> MASSRCPAPRGCRCLPGASLAWLGTVLLLLADWVLLRTALPRIFSLLVPTALPLLRVWAVGLSRWAVLWLGACGVLRATVGSKSENAGAQGWLAALKPLAAALGLALPGLALFRELISWGAPGSADSTRLLHWGSHPTAFVVSYAAALPAAALWHKLGSLWVPGGQGGSGNPVRRLLGCLGSETRRLSLFLVLVVLSSLGEMAIPFFTGRLTDWILQDGSADTFTRNLTLMSILTIASAVLEFVGDGIYNNTMGHVHSHLQGEVFGAVLRQETEFFQQNQTGNIMSRVTEDTSTLSDSLSENLSLFLWYLVRGLCLLGIMLWGSVSLTMVTLITLPLLFLLPKKVGKWYQLLEVQVRESLAKSSQVAIEALSAMPTVRSFANEEGEAQKFREKLQEIKTLNQKEAVAYAVNSWTTSISGMLLKVGILYIGGQLVTSGAVSSGNLVTFVLYQMQFTQAVEVLLSIYPRVQKAVGSSEKIFEYLDRTPRCPPSGLLTPLHLEGLVQFQDVSFAYPNRPDVLVLQGLTFTLRPGEVTALVGPNGSGKSTVAALLQNLYQPTGGQLLLDGKPLPQYEHRYLHRQVAAVGQEPQVFGRSLQENIAYGLTQKPTMEEITAAAVKSGAHSFISGLPQGYDTEVDEAGSQLSGGQRQAVALARALIRKPCVLILDDATSALDANSQLQVEQLLYESPERYSRSVLLITQHLSLVEQADHILFLEGGAIREGGTHQQLMEKKGCYWAMVQAPADAPE;> MRLPDLRPWTSLLLVDAALLWLLQGPLGTLLPQGLPGLWLEGTLRLGGLWGLLKLRGLLGFVGTLLLPLCLATPLTVSLRALVAGASRAPPARVASAPWSWLLVGYGAAGLSWSLWAVLSPPGAQEKEQDQVNNKVLMWRLLKLSRPDLPLLVAAFFFLVLAVLGETLIPHYSGRVIDILGGDFDPHAFASAIFFMCLFSFGSSLSAGCRGGCFTYTMSRINLRIREQLFSSLLRQDLGFFQETKTGELNSRLSSDTTLMSNWLPLNANVLLRSLVKVVGLYGFMLSISPRLTLLSLLHMPFTIAAEKVYNTRHQEVLREI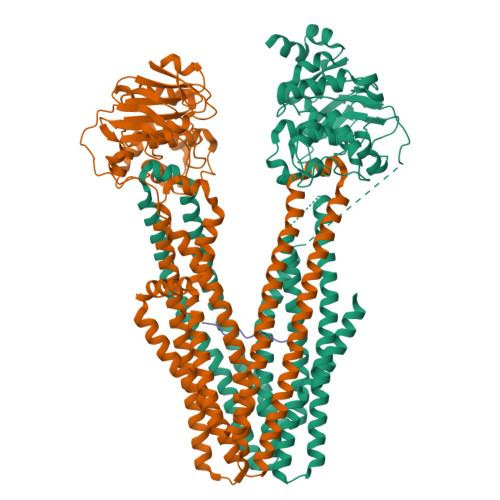QDAVARAGQVVREAVGGLQTVRSFGAEEHEVCRYKEALEQCRQLYWRRDLERALYLLVRRVLHLGVQMLMLSCGLQQMQDGELTQGSLLSFMIYQESVGSYVQTLVYIYGDMLSNVGAAEKVFSYMDRQPNLPSPGTLAPTTLQGVVKFQDVSFAYPNRPDRPVLKGLTFTLRPGEVTALVGPNGSGKSTVAALLQNLYQPTGGQVLLDEKPISQYEHCYLHSQVVSVGQEPVLFSGSVRNNIAYGLQSCEDDKVMAAAQAAHADDFIQEMEHGIYTDVGEKGSQLAAGQKQRLAIARALVRDPRVLILDEATSALDVQCEQALQDWNSRGDRTVLVIAHRLQTVQRAHQILVLQEGKLQKLAQL;> ILKEPVHGV>KAPPLVNLAEEKDVKVTVGENMDLKNADLLTDGDKYYLQHDATGNKEGNNWENYQEQGTEVTSTAEGKNGVWVQVDLGASYPLEVINLKRQVYDGQATIGNGNPSGQGKRLKGTKISYKNTAIVIGNEEDLSDGQIVYYEGNPTLPDGVKQPENVSKPYEEAMGGQWFYMDYANKNGLGATELGTTKEARYIRVYTENPKGAAVKFMELGIYGYENEQDVQSQDGPRRVIDNEHPMMIATAYSNDVYEIGQEEGPELQGSNTVDGRWNAIPDDLKENNVLLLHTNNLRQFAPDHIGQAYLQAFHEHGLQIAYEQGAPIMLLGLTAAATPENGGTQYNITADMDYGWLDLMYRMYPNMQGVFNTENFWAGIHPPCEGSAKMLEIADRFGGFFVWSDQDHGSTVTNIVSNANMKKALEKHGDAFYLIYKNTSSNQPDDLKTSSFFQGSWLAGYTGGWGMLSDTWAWDKQFSKLWQGAGSYNNWQRLCGEPEALLGMQMMSTYLGGGVIYTFEFPEIVYGTSNTNSPANTHVLTELFRYIVNHPAPSKKEIMEETKAVLYGNVSSDFYSGLSGKPTGFQIYETGRYGIIPVIPTWGTRAEVTKKLIQEADKLGVTPPNVLDVKDKNLSGQAKQKYFKDLYPIEYVGNAFADKWEGTWYLYNNKVNTNEKQHAILPLEGEEESARLKVEMEPHEFMIMNESGDGTAMDITLNNYRVNKDEIIFDNKFGLTWTGDFSPGQTTINGKLSVYKYMDEYNVVNAPEGKLSPEDNELRTTTFELTKLAKEPKVQVVKGQQPDTDGQPQYTEPKVEFNEETGKAVITIQTNGWVDLSITGLEFVYDENAQKIEDEP[2x]

We showed by HPAEC-PAD and LC-FD-MS/MS that RgGH98 is specific for blood group A tetrasaccharide type II (BgA II). As expected from the construct, RgGH98 adopts a modular structure with 3 domains. Structural alignment to homologous GH98 enzymes identified the binding pocket and the general acid catalytic residue as Glu 411, which is present in a cleft in the centre of the Cd. Fragmentation of this species showed that the deoxy-hexose was linked to the hexose at the reducing end, as determined by the characteristic fragments at 431 and 449 Da. Together, the HPAEC-PAD and MS/MS analyses confirmed that BgAtri was released from mucin following RgGH98 hydrolysis of the Galβ1-4GlcNAc glycosidic linkage in BgA II.

Incubation of RgGH98 crystals with BgAtri produced a complex with clear electron density for the BgAtri in the binding pocket near Glu 411. RgGH98 makes hydrogen bond interactions with each of the 3 sugar residues present in BgAtri (GalNAcα1-3(Fucα1–2)Gal-): Tyr 289, His 330, and Thr 371 with Fuc; Lys513 with Gal; and Gln 305, Asn 332, and Lys 788 with GalNAc, respectively. No large movements in side chain positions were observed upon ligand binding. The difference between BgA and BgB is the presence of terminal GalNAc and Gal at the nonreducing end of A and B antigens, respectively. Lys 788, present on an extension from the C-term domain, forms part of a hydrogen bonding network with the GalNAc N-acetyl moiety and a ring hydroxyl, forming a stable structure. However, unique to RgGH98, Gln 305 and Trp 528 provide additional interactions, bringing the terminal GalNAc into a location conducive to hydrogen bond with Lys 788. In concert, these residues are proposed, to provide the observed BgA>BgB specificity. Gln 305, Trp 528, and the GalNAc binding site are unique to RgGH98 as compared to Sp3GH98, Sp4GH98, EabC, Cpe0329, and BACOVA_03433. Additional calcium and magnesium ions were modelled in the RgGH98–BgAtri complex and RgGH98 apo crystal structures. However, in these experiments both ions were present at a concentration of 50 mM, increasing the likelihood of nonspecific binding.>SEFVPPPECPVFEPSWEEFTDPLSFIGRIRPLAEKTGICKIRPPKDWQPPFACEVKSFRFTPRVQRLNELEAMTRVRLDFLDQLAKFWELQGSTLKIPVVERKILDLYALSKIVASKGGFEMVTKEKKWSKVGSRLGYLPGKGTGSLLKSHYERILYPYELFQSGVSLMGVQMPNLDLKEKVEPEVLSTDTQTSPEPGTRMNILPKRTRRVKTQSESGDVSRNTELKKLQIFGAGPKVVGLAMGTKDKEDEVTRRRKVTNRSDAFNMQMRQRKGTLSVNFVDLYVCMFCGRGNNEDKLLLCDGCDDSYHTFCLIPPLPDVPKGDWRCPKCVAEECSKPREAFGFEQAVREYTLQSFGEMADNFKSDYFNMPVHMVPTELVEKEFWRLVSSIEEDVIVEYGADISSKDFGSGFPVKDGRRKILPEEEEYALSGWNLNNMPVLEQSVLAHINVDISGMKVPWLYVGMCFSSFCWHIEDHWSYSINYLHWGEPKTWYGVPSHAAEQLEEVMRELAPELFESQPDLLHQLVTIMNPNVLMEHGVPVYRTNQCAGEFVVTFPRAYHSGFNQGYNFAEAVNFCTADWLPIGRQCVNHYRRLRRHCVFSHEELIFKMAADPECLDVGLAAMVCKELTLMTEEETRLRESVVQMGVLMS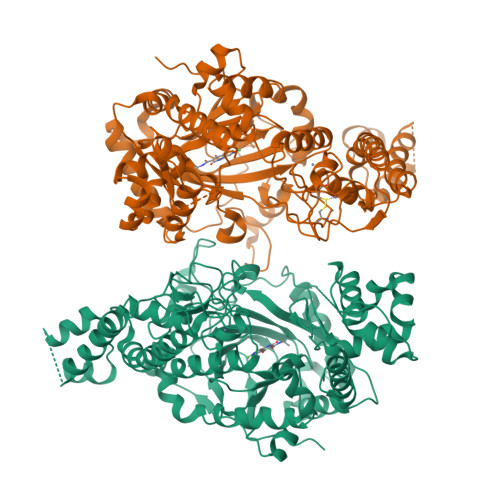EEEVFELVPDDERQCSACRTTCFLSALTCSCNPERLVCLYHPTDLCPCPMQKKCLRYRYPLEDLPSLLYGVKVRAQSYDTWVSRVTEALSANFNHKKDLIELRVMLEDAEDRKYPENDLFRKLRDAVKEAETCASVGNS[2x]>[2x]MLDIHNPATDHHDMRDLTIIGGGPTGIFAAFQCGMNNISCRIIESMPQLGGQLAALYPEKHIYDVAGFPEVPAIDLVESLWAQAERYNPDVVLNETVTKYTKLDDGTFETRTNTGNVYRSRAVLIAAGLGAFEPR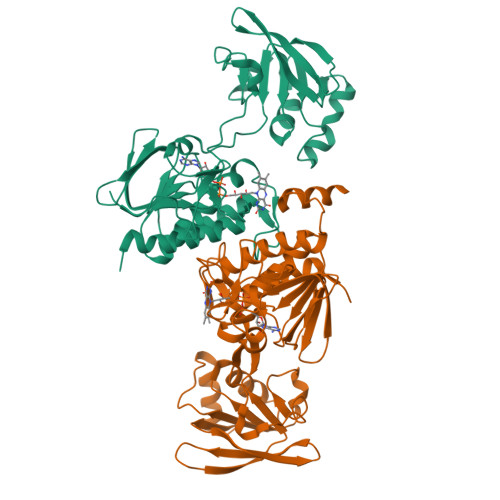KLPQLGNIDHLTGSSVYYAVKSVEDFKGKRVVIVGGGDSALDWTVGLIKNAASVTLVHRGHEFQGHGKTAHEVERARANGTIDVYLETEVASIEESNGVLTRVHLRSSDGSKWTVEADRLLILIGFKSNLGPLARWDLELYENALVVDSHMKTSVDGLYAAGDIAYYPGKLKIIQTGLSEATMAVRHSLSYIKPGEKIRNVFSSVKMAKEKKAAEAGNATENKAE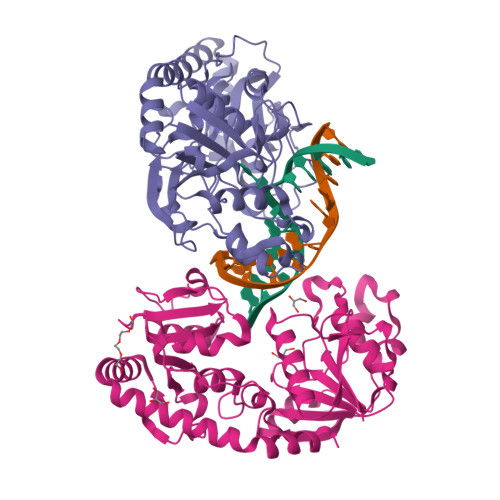>[2x]MKIAIINMGNNVINFKTVPSSETIYLFKVISEMGLNVDIISLKNGVYTKSFDEVDVNDYDRLIVVNSSINFFGGKPNLAILSAQKFMAKYKSKIYYLFTDIRLPFSQSWPNVKNRPWAYLYTEEELLIKSPIKVISQGINLDIAKAAHKKVDNVIEFEYFPIEQYKIHMNDFQLSKPTKKTLDVIYGGSFRSGQRESKMVEFLFDTGLNIEFFGNAREKQFKNPKYPWTKAPVFTGKIPMNMVSEKNSQAIAALIIGDKNYNDNFITLRVWETMASDAVMLIDEEFDTKHRIINDARFYVNNRAELIDRVNELKHSDVLRKEMLSIQHDILNKTRAKKAEWQDAFKKAIDL Voltage-gated K+ channels of the Kv3 family represent an important subfamily among the 70 different Kv channel genes in the human genome, with specialized biophysical properties to sustain high-frequency firing of action potentials. The combination of ultra-fast activation and deactivation kinetics and high activation potential of these channels are key for their ability to repolarize the membrane and terminate the action potential. Like other pore-forming subunits of Kv channels, Kv3 members are comprised of an N-terminal cytoplasmic T1 domain, which is involved but not required for Zn2+-mediated tetramerization, followed by the voltage-sensing domain (VSD) with transmembrane helices S1–S4 which is connected via a helical linker (S4/S5L) to the pore forming domain (PD) of the channel. Here, we present cryo-EM structures of the human Kv3.1a channel in an activated state, providing mechanistic insights into the modulation of Kv3 channels by the cytoplasmic T1 domain.

To elucidate the structural determinants underlying the biophysical properties of Kv3 channels, we purified the shorter α-isoform of Kv3.1 from mammalian cells and determined cryo-EM structures under different sample conditions (apo, Zn2+-containing vs. Zn2+-free). We achieved 3D reconstructions between 3.1 and 3.5 Å for the different conditions, which show only minor differences in the overall structure, and no clear densities for additional Zn2+ sites other than the known sites in the T1 domain16 (see Supplementary discussion). The polar head group of the lipid is stabilized by interactions with the imidazole group of H212 in the S1/S2 linker and backbone interactions with Q409 and M414 in S6. Our maps also show densities in the selectivity filter which likely correspond to K+ ions from the purification buffer.

>MGQGDESERIVINVGGTRHQTHRSTLRTLPGTRLAWLAEPDAHSHFDYDPRADEFFFDRHPGVFAHILNYYRTGKLHCPADVCGPLYEEELAFWGIDETDVEPCCWMTYRQHRDAEEALDSFGGAPLDNSADDADADGPGDSGDGEDELEMTKRLALSDSPDGRPGGFWRRWQPRIWALFEDPYSSRYARYVAFASLFFILVSITTFCLETHERFNPIVNKTEIENVRNGTQVRYYREAETEAFLTYIEGVCVVWFTFEFLMRVIFCPNKVEFIKNSLNIIDFVAILPFYLEVGLSGLSSKAAKDVLGFLRVVRFVRILRIFKLTRHFVGLRVLGHTLRASTNEFLLLIIFLALGVLIFATMIYYAERIGAQPNDPSASEHTHFKNIPIGFWWAVVTMTTLGYGDMYPQTWSGMLVGALCALAGVLTIAMPVPVIVNNFGMYYSLAMAKQKLPKKKKKHIPRPPQLGSPNYCKSVVNSPHHSTQSDTCPLAQEEILEINRAGRKPLRGMSIAENLYFQ[4x]> MQAYSNPGYSSFPSPTGLEPSCKSCGAHFANTARKQTCLDCKKNFCMTCSSQVGNGPRLCLLCQRFRATAFQREELMKMKVKDLRDYLSLHDIS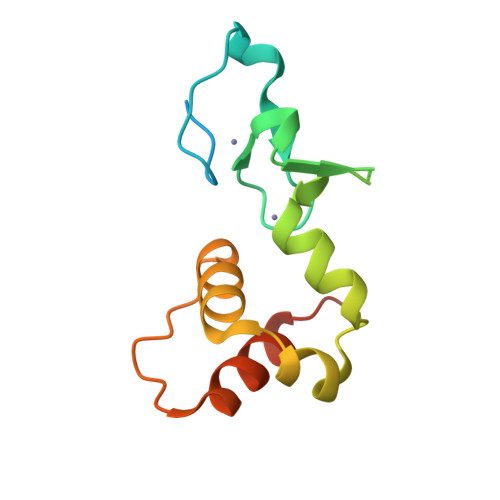TEMCREKEELVLLVLGQQPVISQEDR> KRIVACDDPDFLTSYFAHSRGHHLSAWKANLKDKFLNENIHKYTKITDKDTYIIFHIDFDCFFATVAYLCRSSSFSACDFKRDPIVVCHGTKNSDIASCNYVARSYGIKNGMWVSQAEKMLPNGIKLISLPYTFEQFQLKS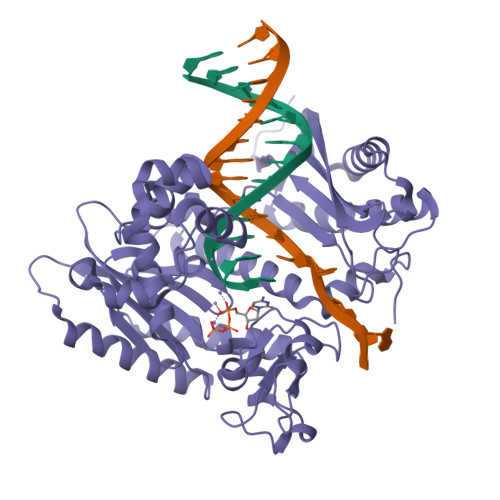EAFYSTLKRLNIFNLILPISIDEAVCVRIIPDNIHNTNTLNARLCEEIRQEIFQGTNGCTVSIGCSDSLVLARLALKMAKPNGYNITFKSNLSEEFWSSFKLDDLPGVGHSTLSRLESTFDSPHSLNDLRKRYTLDALKASVGSKLGMKIHLALQGQDDEESLKILYDPKEVLQRKSLSIDINWGIRFKNITQVDLFIERGCQYLLEKLNEINKTTSQITLKLMRRCKDAPIEPPKYMGMGRCDSFSRSSRLGIPTNEFGIIATEMKSLYRTLGCPPMELRGLALQFNKLVDVGPDNNQLK>[3x]HSSGLVPRGSHMSQERILDGEEDEINHKIFDLKRTLKDNLPLDRDFIDRLKRYFKDPSDQVLALRELLNEKDLTAEQVELLTKIINEIISGSEKSVNAGINSAIQAKLFGNKMKLEPQLLRACYRGFIMGNISTTDQYIEWLGNFGFNHRHTIVNFVEQSLIVDMDSEKPSCNAYEFGFVLSKLIAIKMIRTSDVIFMKKLESSSLLKDGSLSAEQLLLTLLYIFQYPSESEQILTSVIEVSRASHED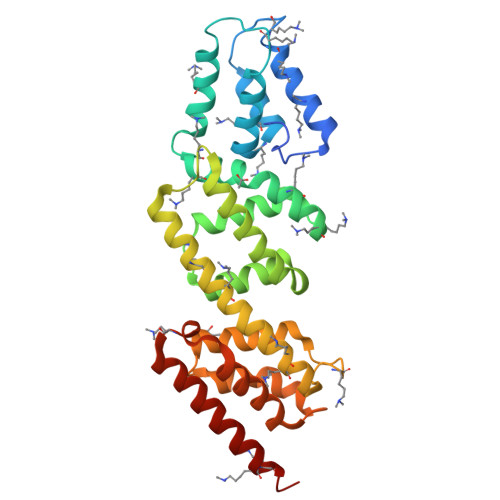SVVYQTYLSSVNESPHDIFKSESEREIAINILRELVTSAYKKELSR>TDTTNSIKHVISPLARQTLQDRDLTRPVAGKRPIRLLPWLQVVKIGGRVMDRGADAILPLVEELRKLLPEHRLLILTGAGVRARHVFSVGLDLGLPVGSLAPLAASEAGQNGHILAAMLASEGVSYVEHPTVADQLAIHLSATRAVVGSAFPPYHHHEFPGSRIPPHRADTGAFLLADAFGAAGLTIVENVDGIYTADPNGPDRGQARFLPETSATDLAK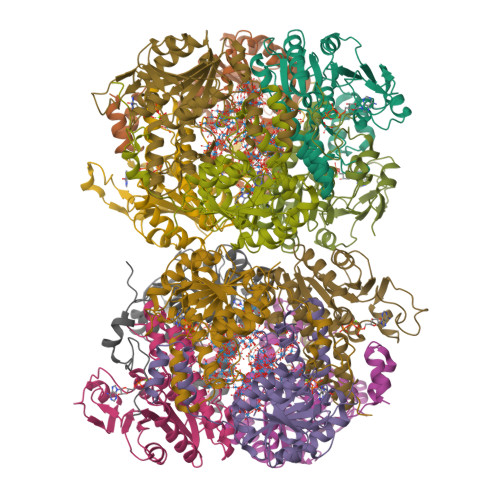SEGPLPVDRALLDVMATARHIERVQVVNGLVPGRLTAALRGEHVGTLIRTGVRPA[6x];>[6x]ANSTAELEELLMQRSLTDPQLQAAAAAAADFRILPDATVIKIGGQSVIDRGRAAVYPLVDEIVAARKNHKLLIGTGAGTRARHLYSIAAGLGLPAGVLAQLGSSVADQNAAMLGQLLAKHGIPVVGGAGLSAVPLSLAEVNAVVFSGMPPYKLWMRPAAEGVIPPYRTDAGCFLLAEQFGCKQMIFVKDEDGLYTANPKTSKDATFIPRISVDEMKAKGLHDSILEFPVLDLLQSAQHVREVQVVNGLVPGNLTRALAGEHVGTIITAS>MDKDEAWKQVEQLRREGATRIAYRSDDWRDLKEAWKKGADILIVSSKADDYRARAAAAAKELGNVKPIVDALLAEAKKARDEAWKQVEQLRREGATEIAYRSDDWRDLKEAWKKGADILIVDATDKNEAWKQVEQLRREGATRIAYRSDDWRDLKEAWKKGADILIVDVNARIEKRRKKLAAEGRTDPAVIEAEAAKAREEGWKQVEQLRREGATEIAYRSDDWRDLKEA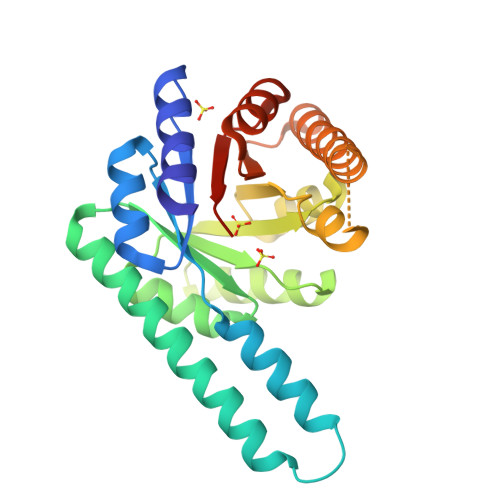WKKGADILIVDATLEHHHHHH[2x]> GAEPYTTIHQPGYCAFYDECGKNPELSGSLMTLSNVSCLSNTPARKITGDHLILLQKICPRLYTGPNTQACCSAKQLVSLEASLSITKALLTRCPACSDNFVNLHCHNTCSPNQSLFINVTRV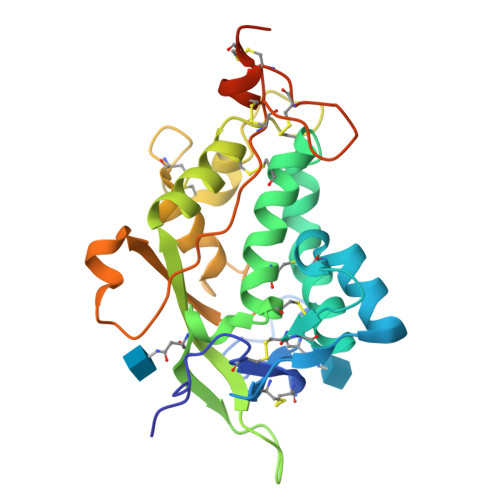AQLGAGQLPAVVAYEAFYQHSFAEQSYDSCSRVRVPAAATLAVGTMCGVYGSALCNAQRWLNFQGDTGNGLAPLDITFHLLEPGQAVGSGIQPLNEGVARCNESQGDDVATCSCQDCAASCPAIARPQALDSTFYLGQMPGS Tripartite α-PFTs are members of the ClyA α-PFT family. Proteins in this family undergo a large scale conformational change from a compact soluble structure, where the hydrophobic residues are hidden often within a β-tongue motif, to an extended pore structure with the hydrophobic residues exposed in two extended α-helices which insert into the cell membrane. Here we show that S. marcescens has a tripartite haemolytic α-PFT (SmhABC), and propose a mechanism of pore assembly. We present the structures of the soluble A component (SmhA), as well as the soluble and pore conformations of the B component (SmhB).

SmhA folds into two distinct domains, a compact five helical bundle (α1, α2, α3, α6 and α7), and an associated head domain containing two helices (α4 and α5), and the β-tongue domain (two long anti-parallel β-strands, β1 and β2). In all monomers, there is missing density for approximately 20 residues between β1 and β2 (G208 – A229). Residues E192-V205 (β1 and loop to α3) and Y231-N250 (β2 and loop to α4) of the β-tongue domain are largely hydrophobic containing only polar uncharged and nonpolar residues, and are buried in the core of the protein, packing against α1, α3, α4, α5 (residues A272-Q283), and residues N351-E367 at the C-terminus. However, in SmhA, NheA and Hbl-B, this region has an additional extended loop and short helix that extends the length of the tail domain, a feature not observed in SmhB or AhlB. AhlB and SmhB use both a short β-strand and a short helix connected by a loop, while SmhA uses only a short loop perpendicular to β1. The second region is between the N-terminus and β-tongue, which includes a family conserved glutamine (Q38 SmhA, Q32 SmhB, Q45 NheA) on the N-terminal helix α1 that forms hydrogen bonds with the β-sheet backbone of the β-tongue. In SmhA Q38 and in NheA Q45 also interact with Q263 and Q282, respectively on α6, a residue conserved in all A component proteins. In addition, both SmhA and SmhB contain a family conserved (conserved in all but 1 sequence) lysine residue at the C-terminus (K333 in both SmhA and SmhB) that forms a hydrogen bond with a conserved hydroxyl (T81 SmhA; T78 SmhB) on helix α2. As soluble SmhA, SmhB and AhlB all share very similar structures, we propose that the head domain of SmhA would also unfold into its pore form about 2 hinges in the same way as seen in SmhB and AhlB, with hinge 1 between α3 and α4, and α5 and α6, and hinge 2 between α4 and β1, and α5 and β2. This would result in the pore form of SmhA having a similar extended helical structure to that of AhlB and SmhB.

>MNNLTSIDLSPQTLMAMHISISSQALLNQSYSNLLLSQQLLTSQSMDPGLTVKIKAYQNQLRQQAQVFKQNTVAELIGLYTKASNFAALVNAVNALYSTEDPQVSQKGAEMVAALSDVAQHYQAAAQAVHTQLQAKREMLEPLMGNFLNVIDAIEQGLNAEAKQQAQTIAELNEAIAKNIQSIADAGFKAGEGVVQLGQSIVAAVPLGPTDKKPKEAPTAPPKPLSDQASYMISGIQAISAGASGAQQAVNELKANYAKLAVAYRALATANALLSVAKSVQAQAQLFVDTYVLTEQRMALLPTEWGKVAEAYLTAAPIINQAGSAAEIKQAKQIISLNAEKWQLFSKSIDNAKANYAGNNILPEVLEHHHHHH[8x]(2S)-4-(4-fluorobenzyl)-N-(3-sulfanylpropyl)piperazine-2-carboxamide 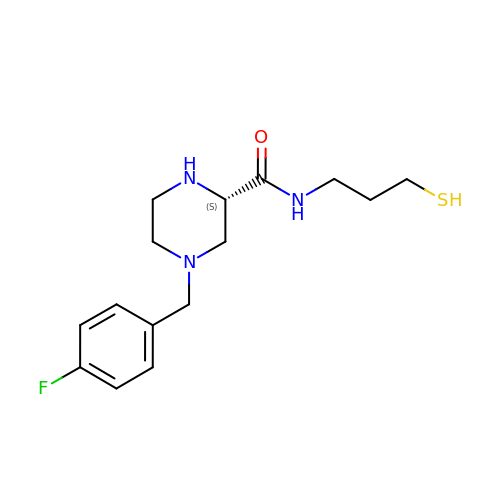| C15 H22 F N3 O S | OYTFYWWLBPDTNS-AWEZNQCLSA-N1-[3-(4-chloro-3,5-dimethylphenoxy)benzyl]-1H-imidazole 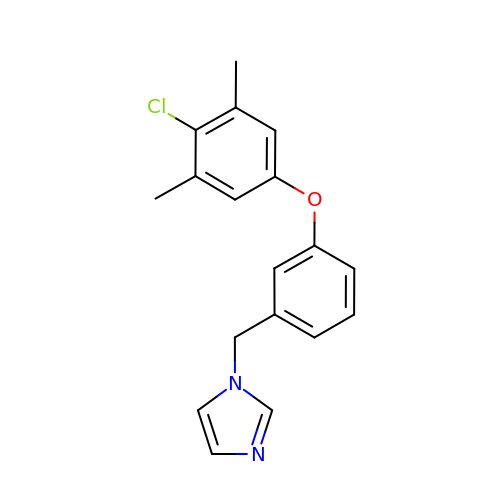| C18 H17 Cl N2 O | KRDUMXYLMIWMMP-UHFFFAOYSA-N Macrophage migration inhibitory factor (MIF) is expressed at high levels in various inflammatory diseases and cancer. Macrophage migration inhibitory factor promotes directional cell migration (or chemotaxis) of various cell types 2, 3, 4. Unlike canonical cytokines and chemokines, a trimeric MIF molecule has three tautomerase active sites at the trimer interfaces 23. Although the enzymatic activity is vestigial, there is accumulating evidence that the active site is important for receptor binding 24, 25.

To structurally verify the proposal for the inhibition of p110γ and p101 expression, we co‐crystallized 1, 2 and 12 with MIF. 1 occupies the bottom half of the catalytic pocket, whereas 2 occupies the upper half. The solvent‐exposed ring structures of 2 and 12 point towards different directions. This suggests that the ring structure of 2 interferes the most with MIF receptor binding with the surrounding residues because 12 is less inhibitory than 2 against the biological activities of MIF. In fact, the solvent‐exposed ring structure of ISO‐1 and 2 are well overlaid. The phenol ring of Tyr36 was moved from the original position (magenta) as shown in 1‐bound structure to a slightly open position (green) in 2‐bound structure, and to the fully open position (light pink) in 12‐bound structure. In contrast, MIF:ISO‐1, MIF:1 and MIF:2 show relatively increased B‐factors (>10 Å2, >30 Å2, and >25 Å2 respectively) for the L2 loop. As MIF:1, MIF:2 and MIF:ISO‐1 inhibited MIF‐induced leucocyte migration and increased B‐factors in L2, it is likely that structural stability of L2 is the critical structural determinant for the chemoattractant activity of MIF. Pro1 attached to 1 revealed the longest displacement (1.9 Å) followed by 4‐IPP (1.1 Å), 2 (0.8 Å), 12 (0.5 Å) and ISO‐1 (0.4 Å). The displacements are 1.1 Å for 1, 0.6 Å for 4‐IPP, 0.6 Å for 2 and 0.5 Å for ISO‐1 and 0.2 Å for 12.

>XMFIVNTNVPRASVPDGFLSELTQQLAQATGKPPQYIAVHVVPDQLMAFGGSSEPCALCSLHSIGKIGGAQNRSYSKLLCGLLAERLRISPDRVYINYYDMNAANVGWNNSTFA[3x]>SVDHGFLVTRHSQTIDDPQCPSGTKILYHGYSLLYVQGNERAHGQDLGTAGSCLRKFSTMPFLFCNINNVCNFASRNDYSYWLSTPEPMPMSMAPITGENIRPFISRCAVCEAPAMVMAVHSQTIQIPPCPSGWSSLWIGYSFVMHTSAGAEGSGQALASPGSCLEEFRSAPFIECHGRGTCNYYANAYSFWLATIERSEMFKKPTPSTLKAGELRTHVSRCQVCMRRT[4x];>[2x]SVSIGYLLVKHSQTDQEPMCPVGMNKLWSGYSLLYFEGQEKAHNQDL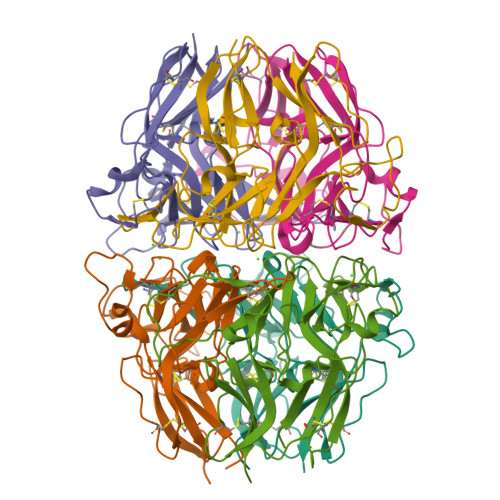GLAGSCLARFSTMPFLYCNPGDVCYYASRNDKSYWLSTTAPLPMMPVAEDEIKPYISRCSVCEAPAIAIAVHSQDVSIPHCPAGWRSLWIGYSFLMHTAAGDEGGGQSLVSPGSCLEDFRATPFIECNGGRGTCHYYANKYSFWLTTIPEQSFQGSPSADTLKAGLIRTHISRCQVCMKNL>SNAMNVSIEEFTHFDFQLVPEPSPLDLVITEPLKNHIEVNGVKSGALLPLPFQTGIGKTYTALNFLLQQMLEQVRSELKEENTGKKSKRLLYYVTDSVDNVVSAKADLLKLIEKQTVKGEPRFTLEQQEYLKAQIVHLPNQSEQLLQCSDAVLNDVLIGFNLNAERDVQAEWSAISGLRRHASNPEVKISLNRQAGYFYRNLIDRLQKKQKGADRVLLSGSLLASVETLLPGEKIRNGSAHVAFLTTSKFLKGFHNTRSRYSPLRDLSGAVLIIDEIDKQNQVILSELCKQQAQDLIWAIRTLRANFRDHQLESSPRYDKIEDLFEPLRERLEEFGTNWNLAFAFNTEGANLNERPVRLFSDRSFTHVSSATHKLSLKSDFLRRKNLIFSDEKVEGSLIEKHGLLTRFVNEADVIYQWFLGTMRKAVFQYWENVRGLEIEVRENRSLEGTFQEAVQSLLTHFNLQEFESAVYESFDTRGLRQSAGGKANKLSSSKSYHHTGLKLVEVAHNQGTRDTVNCKASFLNTSPSGVLADMVDAGAVILGISATARADTVIHNFDFKYLNERLGNKLLSLSREQKQRVNNYYHSRRNYKDNGVVLTVKYLNSRDAFLDALLEEYKPEARSSHFILNHYLGIAESEQAFVRSWLSKLLASIKAFISSPDNRYMLSLLNRTLDTTRQNINDFIQFCCDKWAKEFNVKTKTFFGVNADWMRLVGYDEISKHLNTELGKVVVFSTYASMGAGKNPDYAVNLALEGESLISVADVTYSTQLR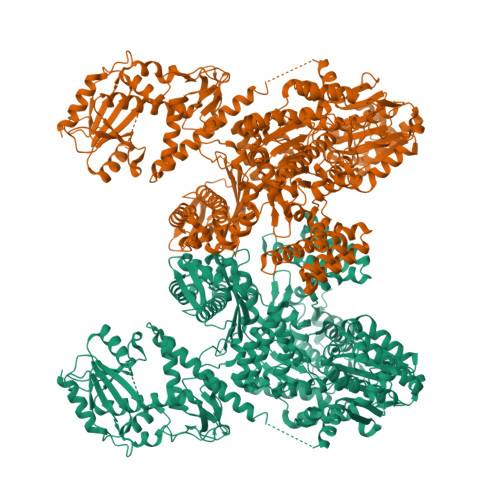SDIDSIYLEKPTQLLLSDDYSHTANQLCQFHQILSLQENGELSPKSAENWCRQQLMGMSRERSLQQYHQTSDYQSAVRKYIEQAVGRAGRTSLKRKQILLFVDSGLKEILAEESRDPSLFSHEYVALVNKAKSAGKSIVEDRAVRRLFNLAQRNNKDGMLSIKALVHRLHNQPASKSDIQEWQDIRTQLLRYPTVAFQPERFNRLYLQSMTKGYYRYQGNLDGDPNSFEFFDRVPYGDMVSEEDCSLATLVQNQYVRPWFERKGFACSWQKEANVMTPIMFTNIYKGALGEQAVEAVLTAFDFTFEEVPNSIYERFDNRVIFAGIEQPIWLDSKYWKHEGNESSEGYSSKIALVEEEFGPSKFIYVNALGDTSKPIRYLNSCFVETSPQLAKVIEIPALIDDSNADTNRTAVQELIKWLHHS[2x]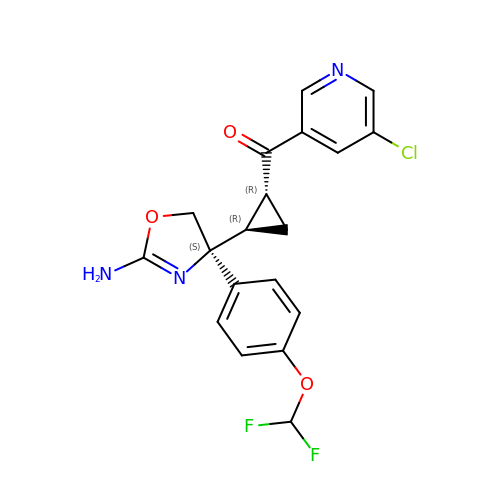[(1~{R},2~{R})-2-[(4~{S})-2-azanyl-4-[4-[bis(fluoranyl)methoxy]phenyl]-5~{H}-1,3-oxazol-4-yl]cyclopropyl]-(5-chloranylpyridin-3-yl)methanone | C19 H16 Cl F2 N3 O3 | AVRZQFKBYKMVDH-SPYBWZPUSA-N>GTAAGCAGCATC[3x];>AGCUUAC[3x];>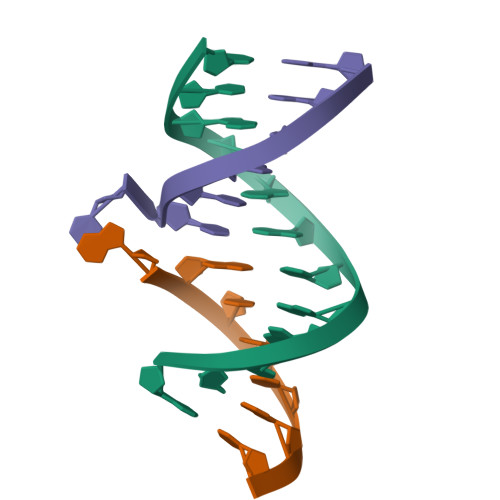GATGCTC[3x]> GIINT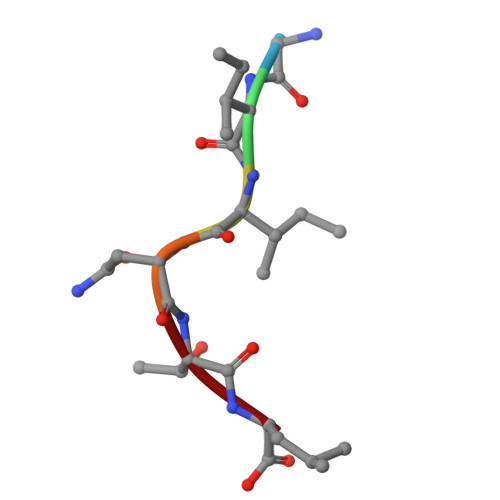L> LPVEKII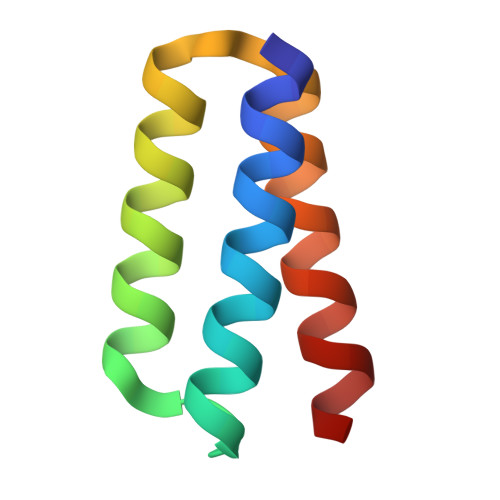REAKKILDELLKRGLIDPELARIAREVLERARKLGNEEAARFVLELIERLRRELS NA is a homotetrameric transmembrane glycoprotein responsible for cleavage of sialic acid from the host cell membrane. By blocking NA enzymatic activity, neuraminidase inhibitors (NAIs) prevent new viral particles from being released from the surface of an infected cell, thus stopping the spread of virus in the airways. In this study, we applied a set of experimental techniques using recombinant NA variants to understand the molecular basis of development of oseltamivir resistance in the viral N1 neuraminidase NA2009. To decipher the structural mechanism of resistance, we determined crystal structures of NA2009 mutants in complex with oseltamivir carboxylate.

Three variants (H275Y, H275Y/I223V, and H275Y/S247N NA2009) crystallized in the monoclinic space group with four molecules in the asymmetric unit, representing the tetrameric biological unit. In enzyme variants containing H275Y in combination with the I223V or S247N mutation, an oseltamivir pose similar to that found in H275Y was observed. The RMSD for superposition of oseltamivir atoms in the H275Y, H275Y/I223V, and H275Y/S247N NA2009 variant was below 0.11 Å. In the H275Y/S247N variant, the water-mediated contact with the oxygen atom between the N247 side-chain and pentyloxy substituent of oseltamivir seen in S247N NA2009 does not form due to the change in position of the pentyloxy substituent caused by the H275Y substitution. The dramatic effect of the H275Y/S247N double mutation on susceptibility to oseltamivir (8-fold and 500-fold increase in Ki compared to the H275Y and S247N single mutants, respectively) can thus be attributed to the combined influence of the change in oseltamivir pose and alterations in the hydration shell structure. Most of the mutated NAs retained Km values almost identical to that of wild-type, while the S247N/H275Y double mutation resulted in a three-fold decrease in substrate-binding ability. Ki values for the I223V/H275Y and S247N/H275Y double mutants were 3900- and 9000-fold higher than the wt NA2009 value, respectively. The catalytic efficiencies of the H275Y, I223V/H275Y, and S247N/ H275Y variants were 4–6% of the wt value, illustrating the significant effect of the H275Y mutation on the enzyme’s catalytic activity.

>SVKLAGNSSLCPVSGWAIYSKDNSVRIGSKGDVFVIREPFISCSPLECRTFFLTQGALLNDKHSNGTIKDRSPYRTLMSCPIGEVPSPYNSRFESVAWSASACHDGINWLTIGISGPDNGAVAVLKYNGIITDTIKSWRNNILRTQESECACVNGSCFTVMTDGPNNGQASYKIFRIEKGKIVKSVEMNAPNYYYEECSCYPDSSEITCVCRDNWHGSNRPWVSFNQNLEYQIGYICSGIFGDNPRPNDKTGSCGPVSSNGANGVKGFSFKYGNGVWIGRTKSISSRNGFEMIWDPNGWTGTDNNFSIKQDIVGINEWSGYSGSFVQHPELTGLDCIRPCFWVELIRGRPKENTIWTSGSSISFCGVNSDTVGWSWPDGAELPFTIDK[4x]>MNWKEFEVFCVTYLNKTYGNKFAKKGESDSTTSDILFTGNNPFYIEAKMPHSQCGQFVLIPNRAEYKFDYSPKNKSEINPYTQKIMQFMSENFSEYANL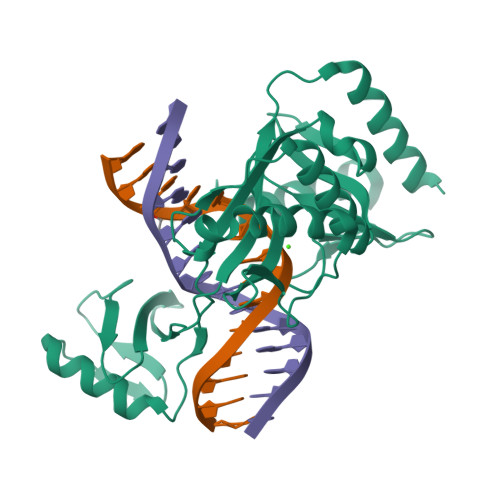STKGKIIPLPESVFVNWIKEYYKSKSVKFFITSNGDFIIFPIEHFEHYFNVSCTYRIKKSGSRHLNSKSLPDFKQALDKKGISYTMRGLELHSDENIHDKRISGDDKDFLIKENNGAYHVKILSNTFNANVIFSISLKNNISLFILNEDRKAFEAAISL[2x]Mammals express three isoforms (α, β and γ) of phosphatidylinositol 5-phosphate 4-kinases (PI5P4Ks), the enzymes that generate phosphatidylinositol bisphosphate (PIP2) from phosphatidylinositol phosphate (PIP), principally via the conversion of PI(5)P to PI(4,5)P2. Variation in catalytic site and putative G-loop sequences may account for the large differences in intrinsic in vitro kinase activity between the isoforms (PI5P4Kα being the most active isoform). More specifically, selective inhibition of PI5P4Kα may also have positive therapeutic effects, as demonstrated by the genetic depletion of PI5P4Kα in p53 null THP-1 cells which resulted in the inhibition of proliferation and also prevented AML development in xenografts. The series was optimised to deliver ARUK2002821 (36), a potent PI5P4Kα inhibitor (pIC50 = 8.0) which is selective vs. other PI5P4K isoforms and has broad selectivity against lipid and protein kinases.

In order to solve a structure of a co-complex of PI5P4Kα with a ligand from this series, a truncated version of human PI5P4Kα was cloned into a bacterial expression vector. There is one PI5P4Kα chain in the asymmetric unit. Overall, the protein structure with 36 bound shows a high degree of similarity with that of the apo structure. However, the Lys228–Thr232 loop segment has a different orientation in the 36 complex, resulting in Leu230 becoming part of the binding pocket. 36 binds deeply in the hydrophobic cleft that forms the ATP binding site in lipid kinases. In particular, the compound binds in the largely hydrophobic pocket formed by Phe134, Ile143, Phe200, Leu230, Leu277 and Ile358. The NH linker in 36 forms a hydrogen bond with the side-chain oxygen acceptor of Asn198, while N1 (see heterocycle numbering in Table 3) of compound 36's pyrrolopyrimidine forms a hydrogen bond with the main-chain nitrogen of Val199. Furthermore, N3 of the pyrrolopyrimidine is seen to make a hydrogen bond interaction with an ordered water in the binding site. This water is positioned by further hydrogen bonding to the side-chain oxygen acceptor of Thr196. The side-chains of Phe134, Asn124, Lys145 and Lys209 have been re-orientated compared with the apo structure. These side-chain re-orientations result in a tight fit of the aniline aromatic ring, with the chlorine contacting the lipophilic part of the Lys209 and Thr232 side chains, as well as Leu230 and Leu277.

> GASDPLLSVLMWGVNHSINELSHVQIPVMLMPDDFKAYSKIKVDNHLFNKENMPSHFKFKEYCPMVFRNLRERFGIDDQDFQNSLTRSAPLPNDSQARSGARFHTSYDKRYIIKTITSEDVAEMHNILKKYHQYIVECHGITLLPQFLGMYRLNVDGVEIYVIVTRNVFSHRLSVYRKYDLKGSTVAREASDKEKAKELPTLKDNDFINEGQKIYIDDNNKKVFLEKLKKDVEFLAQLKLMDYSLLVGIHDVERAEQEEVECEENDGEEEGESDGTHPVGTPPDSPGNTLNSSPPLAPGEFDPNIDVYGIKCHENSPRKEVYFMAIIDILTHYDAKKKAAHAAKTVKHGAGAEISTVNPEQYSKRFLDFIGHILT>[2x]MGSDKIHHHHHHENLYFQGMKVAIMGAGAVGCYYGGMLARAGH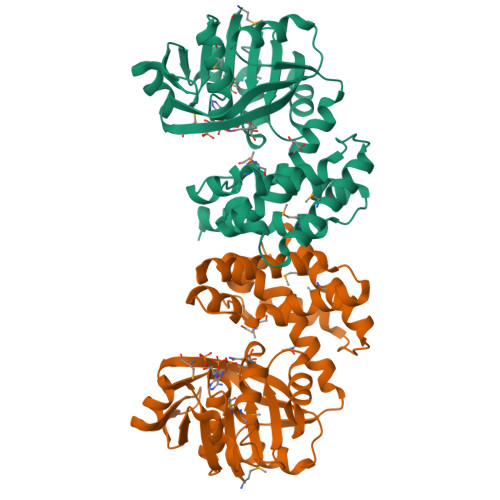EVILIARPQHVQAIEATGLRLETQSFDEQVKVSASSDPSAVQGADLVLFCVKSTDTQSAALAMKPALAKSALVLSLQNGVENADTLRSLLEQEVAAAVVYVATEMAGPGHVRHHGRGELVIEPTSHGANLAAIFAAAGVPVETSDNVRGALWAKLILNCAYNALSAITQLPYGRLVRGEGVEAVMRDVMEECFAVARAEGVKLPDDVALAIRRIAETMPRQSSSTAQDLARGKRSEIDHLNGLIVRRGDALGIPVPANRVLHALVRLIEDKQQHG>GPNVAFDIKAQAKGVDNAEYGNSIMTAKTKPDGSFEFNHDMIDGVKTIGYGKLTGKVNHHYVANKDGSVTAFVDSVTLYKYEYRNVAQNAAVNQNIVFRVLTKDGRPIFEKAHNGNKTFAETLNKTLQLNLKYELKPHASSGNVEVFKIH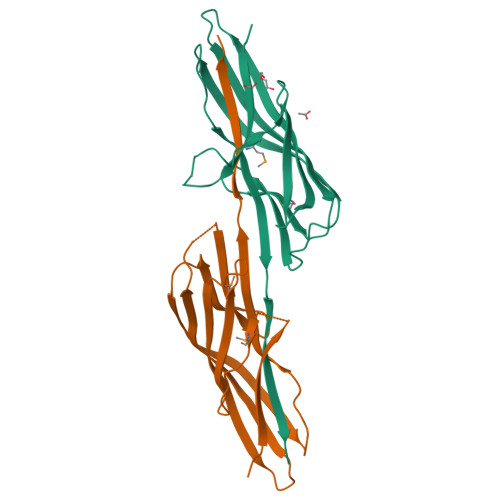DDWVHDTHGSALVSYVNNN[2x]>ADTIVAVELDTYPNTDIGDPNYQHIGINIKSIRSKATTRWNVQDGKVGTAHISYNSVAKRLSAIVSYPGGSSATVSYDVDLNNILPEWVRVGLSASTGLYKETNTILSWSFTSKLKTNSTADAQSLHFTFNQFSQNPKDLILQGDASTDSDGNLQLTRVSNGSPQSNSVGRALYYAPVHV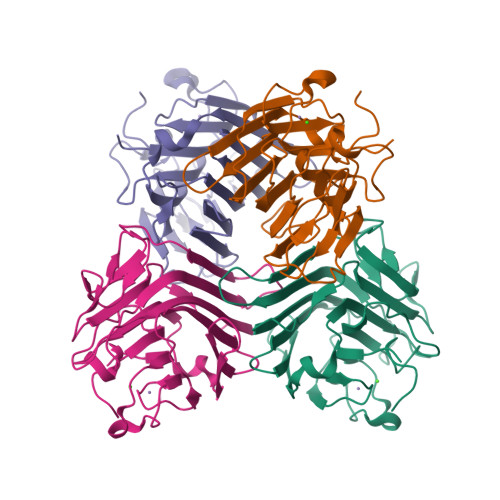WDKSAVVASFDATFTFLIKSTDSDIADGIAFFIANTDSSIPHGSGGRLLGLFPDAN[4x]> GAMDPEFMEMWHEGLEEASRLYFGERNVKG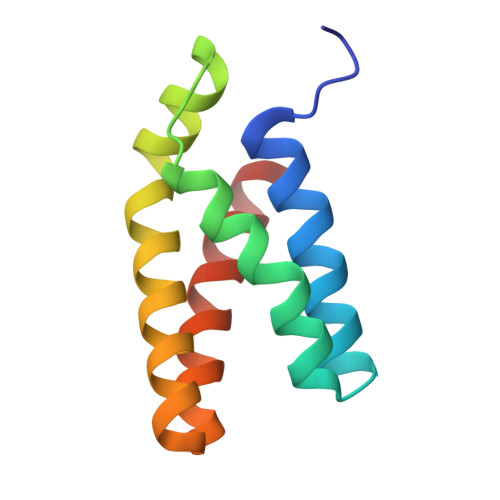MFEVLEPLHAMMERGPQTLKETSFNQAYGRDLMEAQEWCRKYMKSGNVKDLTQAWDLYYHVFRRISKQ> MTKAELRRRARAAWRRLDLKALSRAVGAALLPWLRERGFRHILLYHPLPHELNLLPLMEAYPARYYLPKVAGKGLTVHPFGPLAPGPFGLLEPTTPPEDPRVLDLVVVPGLAFDREGYRLGHGQGFYDRFLKEVRAATVGVVPQALLFPAL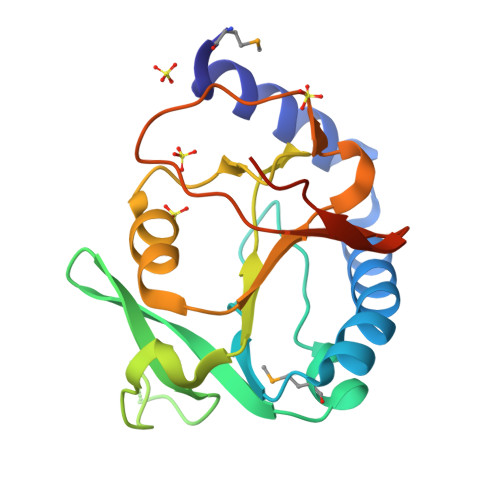PRDPWDVPVDHLATEAGVEAVKRPAPGPGGLLD> AALPQDEKLITGQLDNGLRYMIYPHAHPKDQVNLWLQIHTGSLQEEDNELGVAHFVEHMMFNGTKTWPGNKVIETFESMGLRFGRDVNAYTSYDETVYQVSLPTTQKQNLQQVMAIFSEWSNAATFEKLEVDAERGVITEEWRAHQDAKWRTSQARRPFLLANTRNLDREPIGLMDTVATVTPAQLRQFYQRWYQPNNMTFIVVGDIDSKEALALIKDNLSKLPANKAAENRVWPTKAENHLRFNIINDKENRVNGIALYYRLPMVQVNDEQSFIEQAEWSMLVQLFNQRLQERIQSGELKTISGGTARSVKIAPDYQSLFFRVNARDDNMQDAANALMAELATIDQHGFSAEELDDVKSTRLTWLKNAVDQQAERDLRMLTSRLASSSLNNTPFLSPEETYQLSKRLWQQITVQSLAEKWQQLRKNQDAFWEQMVNNEVAAKKALSPAAILALEKEYANKKLAAYVFPGRNLSLTVDADPQAEISSKETLAENLTSLTLSNGARVILAKSAGEEQKLQIIAVSNKGDLSFPAQQKSLIALANKAVSGSGVGELSSSSLKRWSAENSVTMSSKVSGMNTLLSVSARTNNPEPGFQLINQRITHSTINDNIWASLQNAQIQALKTLDQRPAEKFAQQMYETRYADDRTKLLQENQIAQFTAADALAADRQLFSSPADITFVIVGNVAEDKLVALITRYLGSIKHSDSPLAAGKPLTRATDNASVTVKEQNEPVAQVSQWKRYDSRTPVNLPTRMALDAFNVALAKDLRVNIREQASGAYSVSSRLSVDPQAKDISHLLAFTCQPERHDELLTLANEVMVKRLAKGISEQELNEYQQNVQRSLDIQQRSVQQLANTIVNSLIQYDDPAAWTEQEQLLKQMTVENVNTAVKQYLSHPVNTYTGVLLPKLEHHHHHH

In Pectobacterium, iron acquisition via plant ferredoxin is mediated by the Ferredoxin uptake system (Fus), a molecular machine consisting of inner and outer membrane transporters and a periplasmically localised protease. Intriguingly, the outer membrane transporter from this system, a TonB-dependent transporter (TBDT) designated FusA, imports intact ferredoxin into the periplasm of the bacteria where it is processed by the M16 family protease FusC. To confirm the common architecture of these systems, we characterised the gene cluster analogous to the Fus from Escherichia coli: the ydd/pqqL operon. Furthermore, through structural and biochemical characterisation of the distantly related Fus homologues, YddB and PqqL from E. coli, we show that these proteins share key features with FusA and FusC, suggesting a conserved function.

PqqL was expressed recombinantly, purified and crystallised in order to solve its structure. PqqL consists of two clam-shell like halves, each formed from two M16 protease subunits. This domain structure is analogous to its distant homologue FusC; however, FusC was crystallised in complex with its ferredoxin substrate and adopted a closed clam-shell conformation. In contrast, in the absence of substrate, PqqL adopts an entirely open, highly extended conformation. This domain arrangement has not previously been observed in structures of M16 proteases. In addition to electron density for the PqqL polypeptide chain, density was observed in the predicted peptidase active site of the N-terminal subunit of PqqL, which was attributable to a catalytic metal ion coordinated by histidines 80 and 84. In common with other proteases of this family, these residues form part of the catalytic inverzincin H-x-x-E-H motif in which the two histidine residues coordinate a zinc ion, with the glutamate additionally required for catalysis; this suggests the protein binds a putative Zn ion and serves as a metalloprotease. In order to determine if the crystal structure of PqqL is consistent with its conformation in solution we utilised small angle X-ray scattering (SAXS). In solution, PqqL was found to have maximum dimensions of 140 Å, in good agreement with the 130 Å observed in the crystal structure.>GPLGSVVRAKFNFQQTNEDELSFSKGDVIHVTRVEEGGWWEGTHNGRTGWFPSNYVREI[2x];>PPVIAPR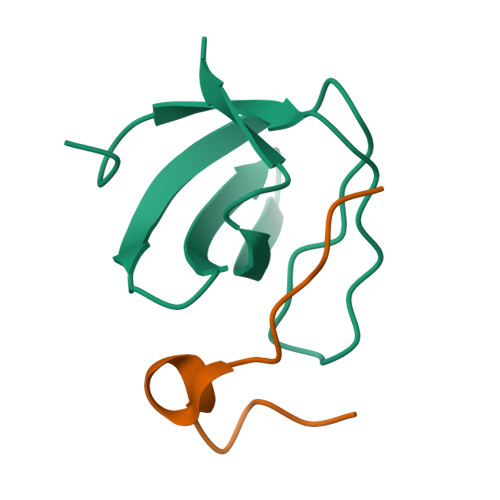PEHTKSIYTRS[2x]> MSRLSEPSPYVEFDRRQWRALRMSTPLALTEEELVGLRGLGEQIDLLEVEEVYLPLARLIHLQVAARQRLFAATAEFLGEPQQNPDRPVPFIIGVAGSVAVGKSTTARVLQALLARWDHHPRVDLVTTDGFLYPNAELQRRNLMHRKGFPESYNRRALMRFVTSVKSGSDYACAPVYSHLHYDIIPGAEQVVRHPDILILEGLNVLQTGPTLMVSDLFDFSLYVDARIEDIEQWYVSRFLAMRTTAFADPESHFHHYAAFSDSQAVVAAREIWRTINRPNLVENILPTRPRATLVLRKDADHSINRLRL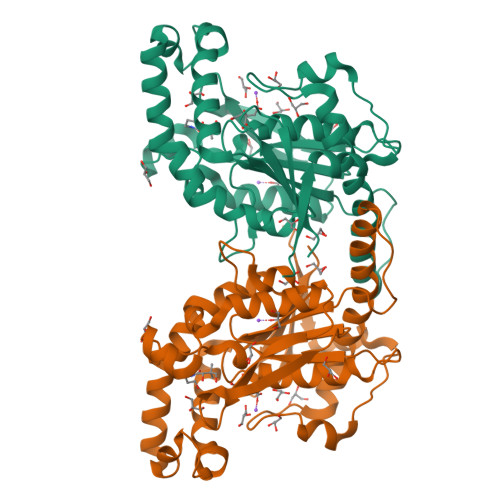RKL> GRTTDPVRMYMREMGTVELLTREGEIDIAKRIEDGINQVQCSVAEYPEAITYLLEQYDRVEAEEARLSDLITGFVDPNAEEDLAPTATHVGSELSQEDLDDDEDEDEEDGDDDSADDDNSIDPELAREKFAELRAQYVVTRDTIKAKGRSHATAQEEILKLSEVFKQFRLVPKQFDYLVNSMRVMMDRVRTQERLIMKLCVEQCKMPKKNFITLFTGNETSDTWFNAAIAMNKPWSEKLHDVSEEVHRALQKLQQIEEETGLTIEQVKDINRRMSIGEAKARRAKKEMVEANL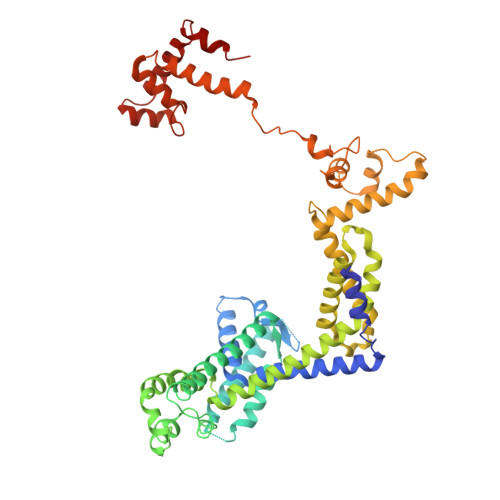RLVISIAKKYTNRGLQFLDLIQEGNIGLMKAVDKFEYRRGYKFSTYATWWIRQAITRSIADQARTIRIPVHMIETINKLNRISRQMLQEMGREPTPEELAERMLMPEDKIRKVLKIAKEPISMETPIGDDEDSHLGDFIEDTTLELPLDSATTESLRAATHDVLAGLTAREAKVLRMRFGIDMNTDYTLEEVGKQFDVTRERIRQIEAKALRKLRHPSRSEVLRSFLDD> MGAQVSTQK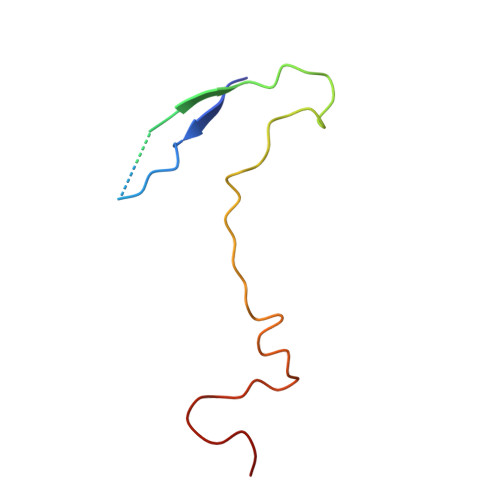TGAHETRLNASGNSIIHYTNINYYKDAASNSANRQDFTQDPGKFTEPVKDIMIKSLPALN>[4x]MSFDDLHKATERAVIQAVDQICDDFEVTPEKLDELTAYFIEQMEKGLAPPKEGHTLASDKGLPMIPAFVTGSPNGTERGVLLAADLGGTNFRICSVNLHGDHTFSMEQMKSKIPDDLLDDENVTSDDLFGFLARRTLAFMKKYHPDELAKGKDAKPMKLGFTFSYPVDQTSLNSGTLIRWTKGFRIADTVGKDVVQLYQEQLSAQGMPMIKVVALTNDTVGTYLSHCYTSDNTDSMTSGEIS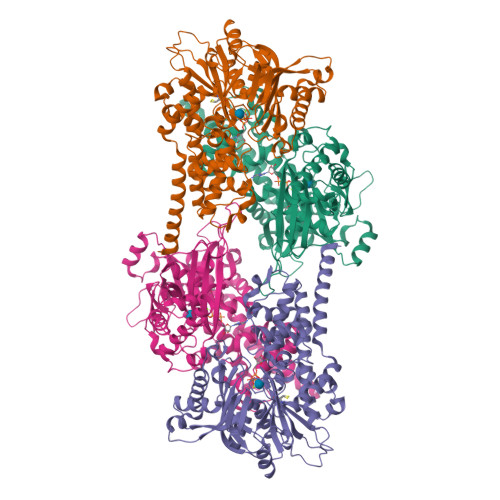EPVIGCIFGTGTNGCYMEEINKITKLPQELRDKLIKEGKTHMIINVEWGSFDNELKHLPTTKYDVVIDQKLSTNPGFHLFEKRVSGMFLGEVLRNILVDLHSQGLLLQQYRSKEQLPRHLTTPFQLSSEVLSHIEIDDSTGLRETELSLLQSLRLPTTPTERVQIQKLVRAISRRSAYLAAVPLAAILIKTNALNKRYHGEVEIGCDGSVVEYYPGFRSMLRHALALSPLGAEGERKVHLKIAKDGSGVGAALCALVA> APLVHHHHHHALANPAICRYPLGMSGGQIPDEDITASSQWSESTAAKYGRLDSEEGDGAWCPEIPVEPDDLKEFLQIDLHTLHFITLVGTQGRHAGGHGIEFAPMYKINYSRDGTRWISWRNRHGKQVLDGNSNPYDIFLKDLEPPIVARFVRFIPVTDHSMNVCMRVELYGCVWLDG;>[3x]XGPPGPPGPPGPRGQPGVLGFPGPPGPPG

The discoidin domain receptors, DDR1 and DDR2, are widely expressed receptor tyrosine kinases that are activated by triple-helical collagen. Binding of triple-helical collagen to DDRs results in slow and sustained receptor phosphorylation (Shrivastava et al., 1997; Vogel et al., 1997), ultimately regulating many aspects of cell proliferation, adhesion, and migration, as well as remodeling of the extracellular matrix (Vogel et al., 2006). Structurally, the DDRs are characterized by an extracellular region consisting of a discoidin (DS) domain that is followed by a domain unique to DDRs, a transmembrane helix, a large cytoplamic juxtamembrane region, and, finally, a C-terminal kinase domain. The major DDR2-binding site in collagens I–III is a GVMGFO motif (O is hydroxyproline) that also binds the matricellular protein SPARC.

Diffraction data to 1.6 Å resolution were collected using synchrotron radiation and the structure of the DDR2 DS-collagen peptide complex was solved by molecular replacement. The DDR2 DS domain is an eight-stranded β-barrel arranged in two antiparallel β sheets (Ichikawa et al., 2007). At the top of the barrel, five protruding loops (L1–L3 connecting β1 to β2, L4 connecting β3 to β4, and L6 connecting β7 to β8) create a trench that accommodates the collagen peptide; the disulfide bridge between Cys73 and Cys177 lies at the bottom of this trench. The DDR2 DS domain interacts with two of the three GVNleGFO motifs in the C-terminal part of the 80 Å–long collagen peptide, burying 530 Å2 of solvent-accessible collagen surface with good shape complementarity (surface complementarity score, 0.71; program SC) (CCP4, 1994). In the DDR2 DS-collagen structure, the leading and middle chains of the collagen peptide (for a definition, see Emsley et al., 2000) account for 40% and 60% of the interface, respectively; the trailing chain is not involved in DDR2 binding. The central feature of the DDR2-collagen interface is an amphiphilic pocket at the top of the DS domain that accommodates Nle21 (leading chain) and Phe23 (middle chain) (for consistency we use the same numbering scheme for the collagen peptide as in our previous work on SPARC; Hohenester et al., 2008). One wall and the floor of the pocket are essentially apolar (Trp52, Thr56, and Cys73-Cys177 disulfide bridge), whereas the other wall is dominated by three charged residues (Asp69, Arg105, and Glu113) interacting with a string of water molecules. A salt bridge between Arg105 and Glu113 forms two hydrogen bonds with the hydroxyl group of Hyp24 (leading chain) and contacts one edge of the phenyl ring of Phe23 (middle chain), suggestive of a C-H⋯π hydrogen bond (Brandl et al., 2001). A comparison of our complex structure with the NMR ensemble of the free DS domain shows that collagen binding leads to a restructuring of loops L1 (bearing the critical Trp52) and L4 (bearing at its base Arg105 and Glu113).>[2x]MSLRAQTAPGRWDGVAVMPYKQTAEAPFQDVSRQLLFADPNLACEWRYFEVDEGGY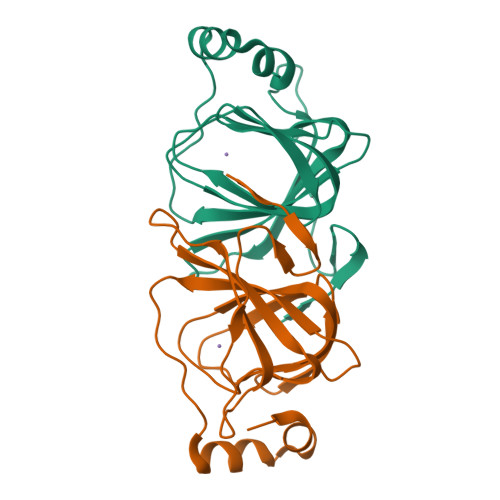STLERHAHVHAVMIHRGHGQCLVGETISDVAQGDLVFIPPMTWHQFRANRGDCLGFLCVVNAARDRPQLPTADDLAELRKDERIADFIRTGGEGHHHHHH>GAMEDKVDAIREAIARNPQEIFQYVRLSQVKRDDKVLGYRVSPGKDPVLFESIGLQ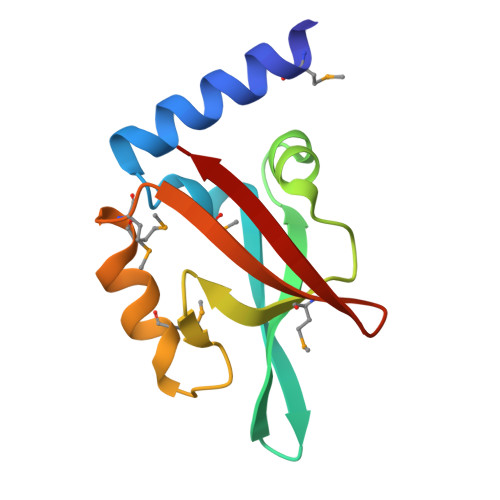DGDMAVALNGLDLTDPNVMNTLFQSMNEMTEMSLTVERDGQQHDVYIQF[2x]> QDSTSDLIPAPPLSKVPLQQNFQDNQFHGKWYVVGKAGNHDLREDKDPRKMQATIYELKEDKSYNVTNVRFVHKKCNYRIWTFVPGSQPGEFTLGNIKSWPGLTSWLVRVVSTNYNQHAMV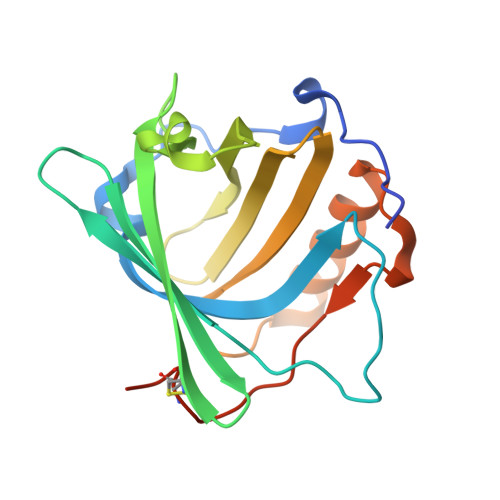FFKRVYQNRELFEITLYGRTKELTNELKENFIRFSKSLGLPENHIVFPVPIDQCIDGSAWSHPQFEK>[9x]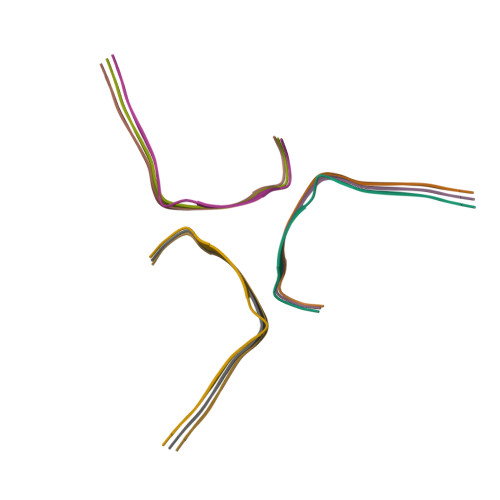GLFDIIKKVASVIGGL>[2x]CGCGAATU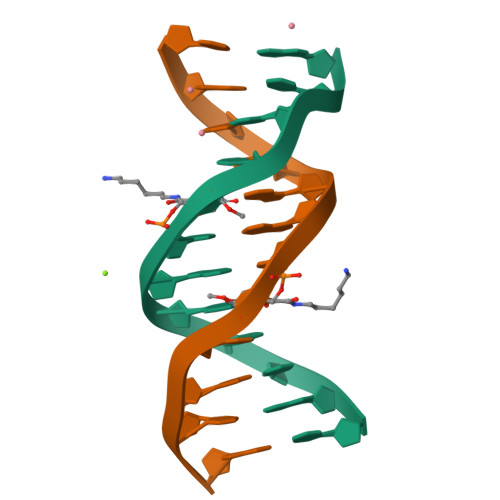CGCG tert-butyl 4-(2-{3-(4-chloro-3-iodophenyl)-1-[3-(morpholin-4-yl)propyl]-1,4,6,7-tetrahydro-5H-pyrazolo[4,3-c]pyridin-5-yl}-2-oxoethyl)piperidine-1-carboxylate 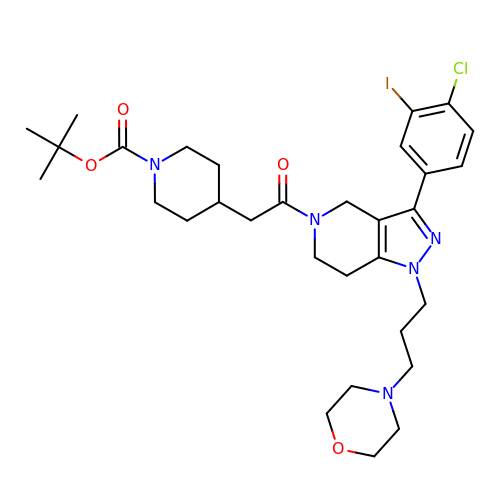| C31 H43 Cl I N5 O4 | ZBMNZIVATWUSMD-UHFFFAOYSA-N> SGSAGNGLVPSDPVLAETMKNERVVQDHNSALRGARPIN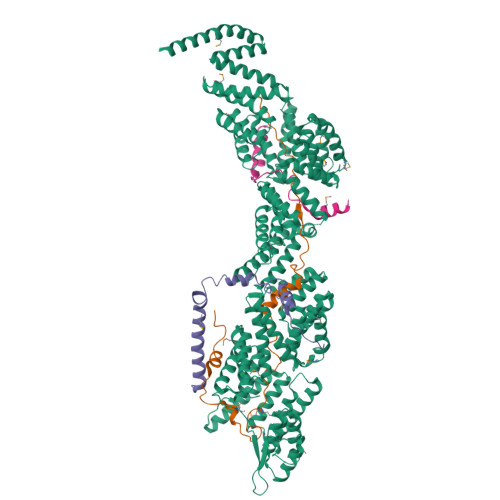FGYLIKDAELKLVQSIKGSLRGSKLPPGHKGAHGRVSKTNGS;> MANTIKVEGYPSMEWPTSLDIPLKASEELVGIDLETDLPDDPTDLKTLLVEESSEKEHWLTIALAYCNHGKTNEGIRLIEMALDVFQNSERASLHTFLTWAHLNLAKGHSLSVETKEHELTQAELNLKDAIGFDPTWIGNMLATVELYYQRGHYDKALETSDLFVKSIHAEDHRSGRQSKPNCLFLLLRAKLLYQKKNYVASLKIFQELLVINPVLQPDPRIGIGLCFWQLKDPKMAIKSWQRALQINSKNTSASILVLLGEFHNSLTDSTNDEVFKETFSKALSDLKNIFSENQNNPVLLTLLQTYHYFKGDFQTVLDIYHHKILKMSPLIAKTVLSESSFWCGRAHYALGDYRKSFIMFQESLKKNEDNLMARLGLGQTQIKSNLLEESIITFENLYKTNESLQELNYILGLLYAGKTLDVKTSKSIPAKELNKLNEKALQYLERYIKLTVAKKNQLIISRVYLVISQLYESQNQYKISLDFLSKALEEMEFVNKDEVPLEILNNLACYHFINGDLTKADNLFEQAKAKVSDMNKSVNITLEYNIARTSEKTNWEKSESIYSQITSSHPSYISARIRNLYIKFAHSKINDSEMNIEINGLLEMNKSDLEMRSFYGWYLKNSEERKNSEKSTSHNKETLVKYNSHDAYALISLANLYVTIARDGKKSRNPKEQEKSKHSYLKAIQLYQKVLQIDPFNVFAAQGVAIIFAESKRLGPALEILRKIRDSLDNEDVQLNLAHCLLEMREFGKAIENYELVLKKFDNERTRPHILNLLGRAWYSRGMKERSVSFFQKALENAKTALELFVQQSAKNKFIHSVKFNIALLQFQIAETLRRSNPKFRTVQQIKDSLEGLEEGLALFKELNDLKEFNMIPKEELEQRIQLGETTMKSALERSLNEQEEFEKDQ;> SMSKKQEYIAPIKYQNSLPVPQLPPKLLAYPEAPETNPDSSQLINSLYVKTNISNLIQQDEDLGMPVDLMKFPGLLNKLDSKLLYGFDNVKLDKDDRILLRDPRIDRLTKT;> SKSDPFSRLKTRTKVYYQEIQKEENAKAKEMAQQEKLQEDRETKERREKELLLAQFRRLGGLERMIGELDIKFDFKF2',3'-DEHYDRO-2',3'-DEOXY-THYMIDINE 5'-TRIPHOSPHATE | 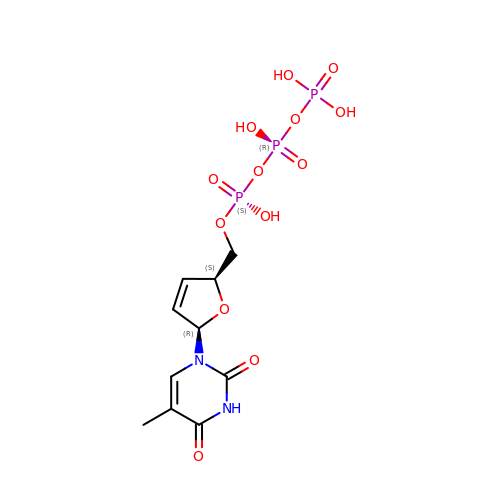C10 H15 N2 O13 P3 | ODSQODTUNULBHF-JGVFFNPUSA-N> QEGLDFPEYDGVDRVINVNAKNYKNVFKKYEVLALLYHEPPEDDKASQRQFEMEELILELAAQVL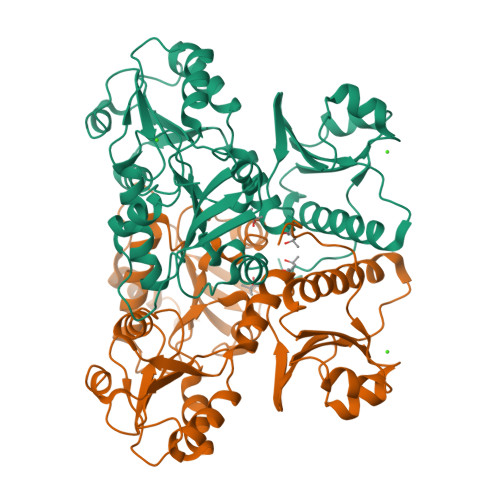EDKGVGFGLVDSEKDAAVAKKLGLTEVDSMYVFKGDEVIEYDGEFSADTIVEFLLDVLEDPVELIEGERELQAFENIEDEIKLIGYFKSKDSEHYKAFEDAAEEFHPYIPFFATFDSKVAKKLTLKLNEIDFYEAFMEEPVTIPGKPNSEEEIVNFVEEHRRSTLRKLKPESMYETWEDDMDGIHIVAFAEEADPDGFEFLETLKAVAQDNTENPDLSIIWIDPDDFPLLVPYWEKTFDIDLSAPQIGVVNVTDADSVWMEMDDEEDLPSAEELEDWLEDVLEGEINTEDDDDDDDD>MAGFLKVVQLLAKYGSKAVQWAWANKGKILDWLNAGQAIDWVVSKIKQILGIK[4x]

Tryptophan is frequently found on the surface of membrane-associated proteins that interact with the lipid membrane. Here, we describe the use of racemic protein crystallography to probe dedicated tryptophan interactions of a model tryptophan-rich bacteriocin aureocin A53 (AucA) by inclusion and/or exclusion of potential ligands. When proteins of natural L-chirality are introduced with their synthetic D-enantiomers, they can form centrosymmetric crystals in achiral space groups with high dimensionality, thereby enabling structures solved at a high resolution over wide-ranging conditions. Finally, in complementation to recent studies, this work illustrates racemic protein crystallography is an effective approach to elucidate tryptophan interactions of membrane-associating proteins.

Testing if the insights obtained from the study of AucA can be transferred to improve our understanding of other bacteriocins, we prepared a distant homolog, lacticin Q (LnqQ), for analysis (48% homology). A synthetic scheme based on chemical ligation was developed and the structure of LnqQ was solved by racemic protein crystallography (0.96 Å). However, LnqQ lacks the corresponding W3 residue and, as anticipated, was found to be monomeric: sharing essentially the same retention time as that of AucA-W3L in the SEC analysis. Indeed, the monomeric L-LnqQ appeared to be more sensitive to proteolytic degradation, as its enantiomeric D-counterpart is resistant to proteolytic degradation and is significantly more potent leading up to 16-fold of difference in activity. Furthermore, W41, which is equivalent to W40 in AucA, is anticipated to be most crucial for activity, and its replacement by a leucine residue nearly demolished all LnqQ’s antibacterial activity likely due to a lack of H-bond donation. For other tryptophan residues including W21, W23 and W32, their replacement resulted in a greater loss in LnqQ’s antibacterial activity, when compared to those of AucA. A plausible explanation is that the LnqQ is more sensitive to residue substitutions because of its monomeric nature, and so for future work the biophysical properties of LnqQ will be investigated. The involving residues, particularly W40 and Lys44, are highly conserved, with presence in lacticin Q25, lacticin Z40 and epidermicin NI0141.>[2x]GPLGSPEFSRTSVQTEDDQLIAGQSARAIMAQLPQEQKAKIAEQVASFQEEKSKLDAEVSKWDDSGNDIIVLAKQMCMIMMEMTDFTRGKGPLKNTSDVISAAKKIAEAGSRMDKLGRTIADHCPDSACKQDLL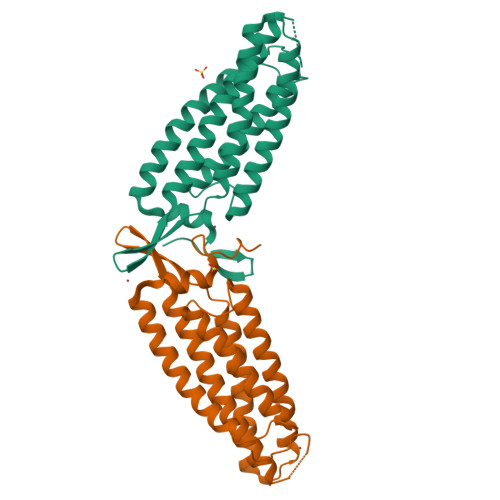AYLQRIALYCHQLNICSKVKAEVQNLGGELVVSGVDSAMSLIQAAKNLMNAVVQTVKASYVASTKYQKSQGMASLNLPAVSWKMKAPEKKPLVKREKQDETQTKIKRASQKKHVNPVQALSEFKAMDSI(2R)-sulfonatepropionyl-CoA | 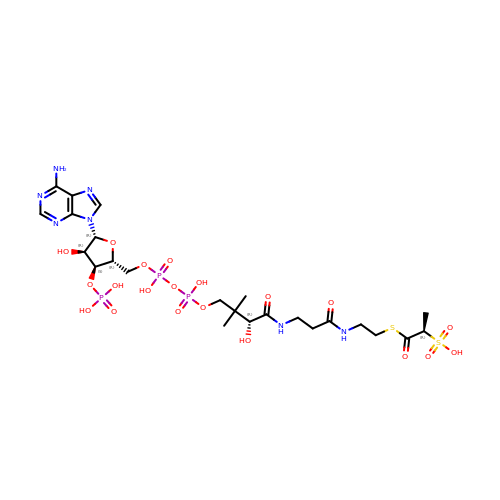C24 H40 N7 O20 P3 S2 | GJGCZNMXHKQRSE-AGCMQPJKSA-N> WSAGDKHKEGVNSHLWIVNRAIDIMSRNTTLVKQDRVAQLNEWRTELENGIYAADYENPYYDNSTFASHFYDPDNGKTYIPFAKQAKETGAKYFKLAGESYKNKDMKQAFFYLGLSLHYLGDVNQPMHAANFTNLSYPQGFHSKYENF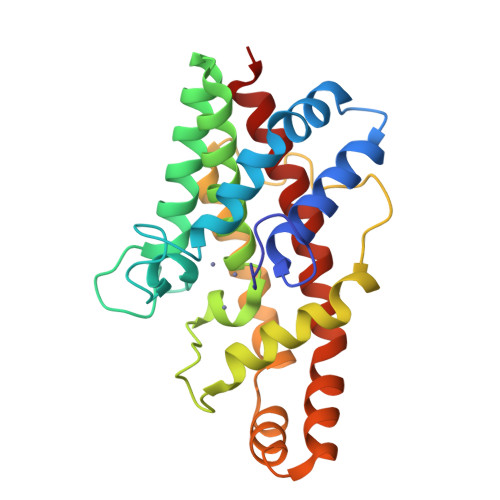VDTIKDNYKVTDGNGYWNWKGTNPEEWIHGAAVVAKQDYSGIVNDNTKDWFVKAAVSQEYADKWRAEVTPMTGKRLMDAQRVTAGYIQLWFDTYGDR The flavoenzymes provide an interesting example whereby very few deposited structures have had their redox states verified during or after data collection. The ‘butterfly bend’ of the flavin (the dihedral angle between the planes formed by the pyrimidine and benzene rings of the isoalloxazine moiety) depends on the oxidation state, with the oxidized form being flat and reduction inducing a bend along the N5–N10 axis. Any discussion of enzyme mechanism deduced from the structure clearly needs to be in the context of the oxidation state observed. Furthermore, X-ray irradiation, through photoelectronic effects, will perturb the redox state in the crystal.

The photoreduction of the flavin in an FMN-containing enzyme during X-ray data collection was followed by Røhr et al., showing the flavin bend. We also observed this effect in crystals of PETN reductase; Fig. 3 shows the difference between the yellow colour of the oxidized enzyme and the colourless X-ray reduced form, and the spectra from the two crystal states. By monitoring the crystal spectrum after varying X-rays doses we were able to use a multi-crystal strategy to obtain a minimally reduced structure and compare this with the X-ray reduced structure, showing clearly that caution is required when interpreting structures that have not been validated with spectroscopy. If the spectrum from the crystal (or irradiated portion of the crystal) is monitored during data collection, it becomes possible to be confident of the redox state of the structure being determined. There are many examples of structures in the PDB that are described as having a particular oxidation state but have most probably been reduced to a greater or lesser extent during data collection.

> AEKLFTPLKVGAVTAPNRVFMAPLTRLRSIEPGDIPTPLMGEYYRQRASAGLIISEATQISAQAKGYAGAPGLHSPEQIAAWKKITAGVHAEDGRIAVQLWHTGRISHSSIQPGGQAPVSASALNANTRTSLRDENGNAIRVDTTTPRALELDEIPGIVNDFRQAVANAREAGFDLVELHSAHGYLLHQFLSPSSNQRTDQYGGSVENRARLVLEVVDAVCNEWSADRIGIRVSPIGTFQNVDNGPNEEADALYLIEELAKRGIAYLHMSETDLAGGKPYSEAFRQKVRERFHGVIIGAGAYTAEKAEDLIGKGLIDAVAFGRDYIANPDLVARLQKKAELNPQRPESFYGGGAEGYTDYPSL> MTSVNSAEASTGAGGGSSNPVKSMWSEGATFSANSVTCTFSRQFLIPYDPEHHYKVFSPAASSCHNASGKEAKVCTITPIMGYST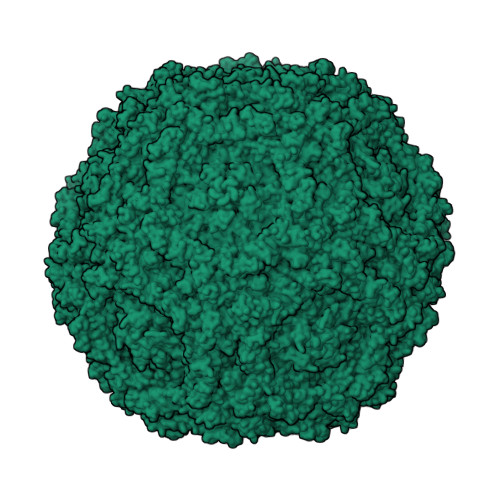PWRYLDFNALNLFFSPLEFQHLIENYGSIAPDALTVTISEIAVKDVTDKTGGGVQVTDSATGRLCMLVDHEYKYPYVLGQGQDTLAPELPIWVYFPPQYAYLTVGDVNTQGISGDSKKLASEESAFYVLEHSSFQLLGTGGTATMSYKFPPVPPENLEGCSQHFYEMYNPLYGSRLGVPDTLGGDPKFRSLTHEDHAIQPQNFMPGPLVNSVSTKEGDSSNTGAGKALTGLSTGTSQNTRISLRPGPVSQPYHHWDTDKYVTGINAISHGQTTYGNAEDKEYQQGVGRFPNEKEQLKQLQGLNMHTYFPNKGTQQYTDQIERPLMVGSVWNRRALHYESQLWSKIPNLDDSFKTQFAALGGWGLHQPPPQIFLKILPQSGPIGGIKSMGITTLVQYAVGIMTVTMTFKLGPRKATGRWNPQPGVYPPHAAGHLPYVLYDPTATDAKQHHRHGYEKPEELWTAKSRVHPL> MMQLDTYDGTLELAGITLGTATTREMLIKGSRLWEGWPEKSDGRTTSYRTIISTKKEKAGDIYIIADFSGAFITDAVLCSWR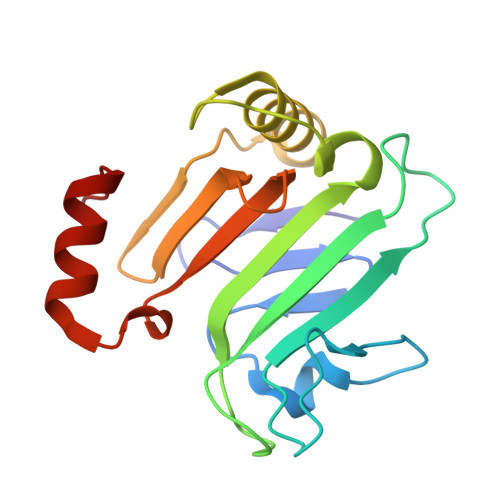FAPEKLMMGIQKKVEGAITKNLRTWFYEKTHIQLPVSGSWGHIDAAYDPHNLTGTIVCNYRSAFHTEDEWRKYCKRNNIIY>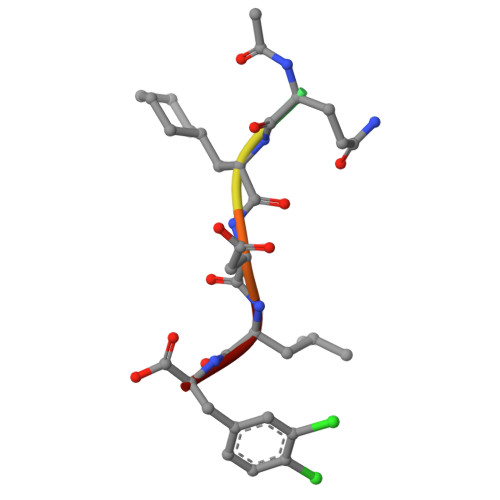 XQADLF> RPPNIVLIFADDLGYGDLGCYGHPSSTTPNLDQLAAGGLRFTDFYVPVSLSTPSRAALLTGRLPVRMGMYPGVLVPSSRGGLPLEEVTVAEVLAARGYLTGMAGKWHLGVGPEGAFLPPHQGFHRFLGIPYSHDQGPCQNLTCFPPATPCDGGCDQGLVPIPLLANLSVEAQPPWLPGLEARYMAFAHDLMADAQREDRPFFLYYASHHTHYPQFSGQSFAERSGRGPFGDSLMELDAAVGTLMTAIGD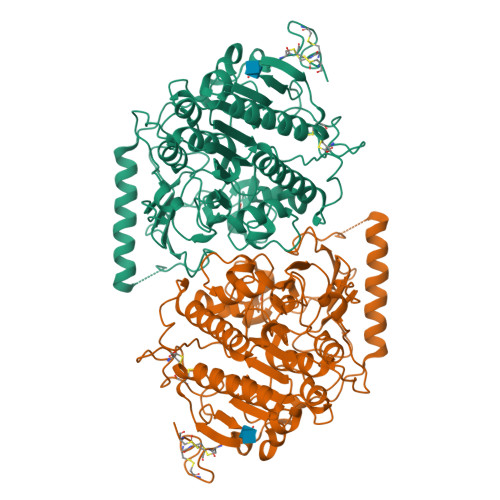LGLLEETLVIFTADNGPETMRMSRGGCSGLLRCGKGTTYEGGVREPALAFWPGHIAPGVTHELASSLDLLPTLAALAGAPLPNVTLDGFDLSPLLLGTGKSPRQSLFFYPSYPDEVRGVFAVRTGKYKAHFFTQGSAHSDTTADPACHASSSLTAHEPPLLYDLSKDPGENYNLLGGVAGATPEVLQALKQLQLLKAQLDAAVTFGPSQVARGEDPALQICCHPGCTPRPACCHCPDPHA>MHHHHHHGYKMVNPPRVVGNWTPKDLSFEYKDVEITTEDNVKLSGWWIDNGSDKTVIPLHGYTSSRWAEHYMRPVIEFLLKEGYNVL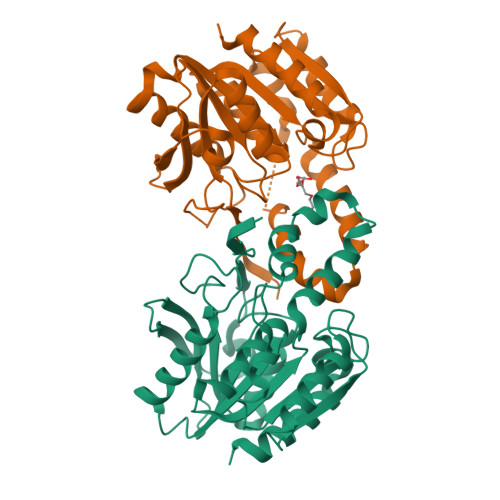AFDFRAHGKSGGKYTTVGDKEILDLKAGVKWLKDNYPEKSKRIGVIGFSMGALVAIRGLSEVKEICCGVADSPPIYLDKTGARGMKYFAKLPEWLYSFVKPFSELFSGGRPINVLNYTNSIKKPLFLIIGRRDTLVKVEEVQEFYERNKHVNPNVELWVTDAPHVRTIQVFPEEWKSRVGEFLKRWMG[4x]>[2x]MVTVGNYCEAEGPVGPAWMQDGLSPCFFFTLVPSTRMALGTLALVLALPCRRRERPAGADSLSWGAGPRISPYVLQLLLATLQAALPLAGLAGRVGTARGAPLPSYLLLASVLESLAGACGLWLLVVERSQARQRLAMGIWIKFRHSPGLLLLWTVAFAAENLALVSWNSPQWWWARADLGQQVQFSLWVLRYVVSGGLFVLGLWAPGLRPQSYTLQVHEEDQDVERSQVRSAAQQSTWR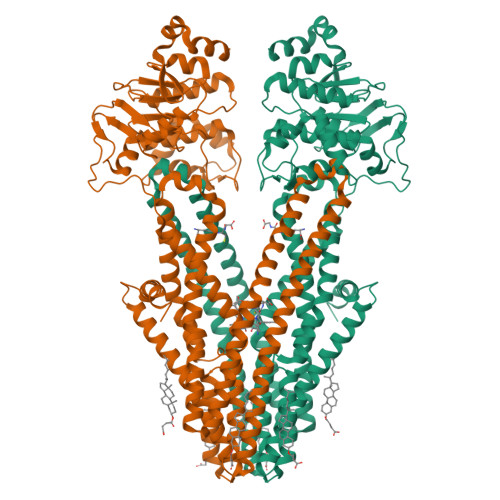DFGRKLRLLSGYLWPRGSPALQLVVLICLGLMGLERALNVLVPIFYRNIVNLLTEKAPWNSLAWTVTSYVFLKFLQGGGTGSTGFVSNLRTFLWIRVQQFTSRRVELLIFSHLHELSLRWHLGRRTGEVLRIADRGTSSVTGLLSYLVFNVIPTLADIIIGIIYFSMFFNAWFGLIVFLCMSLYLTLTIVVTEWRTKFRRAMNTQENATRARAVDSLLNFETVKYYNAESYEVERYREAIIKYQGLEWKSSASLVLLNQTQNLVIGLGLLAGSLLCAYFVTEQKLQVGDYVLFGTYIIQLYMPLNWFGTYYRMIQTNFIDMENMFDLLKEETEVKDLPGAGPLRFQKGRIEFENVHFSYADGRETLQDVSFTVMPGQTLALVGPSGAGKSTILRLLFRFYDISSGCIRIDGQDISQVTQASLRSHIGVVPQDTVLFNDTIADNIRYGRVTAGNDEVEAAAQAAGIHDAIMAFPEGYRTQVGERGLKLSGGEKQRVAIARTILKAPGIILLDEATSALDTSNERAIQASLAKVCANRTTIVVAHRLSTVVNADQILVIKDGCIVERGRHEALLSRGGVYADMWQLQQGQEETSEDTKPQTMER>MKFTVEREHLLKPLQQVSGPLGGRPTLPILGNLLLQVADGTLSLTGTDLEMEMVARVALVQPHEPGATTVPARKFFDICRGLPEGAEIAVQLEGERMLVRSGRSRFSLSTLPAADFPNLDDWQSEVEFTLPQATMKRLIEATQFSMAHQDVRYYLNGMLFETEGEELRTVATDGHRLAVCSMPIGQSLPSHSVIVPRKGVIELMRMLDGGDNPLRVQIGSNNIRAHVGDFIFTSKLVDGRFPDYRRVLPKNPDKHLEAGCDLLKQAFARAAAASNEKFRGVRLYVSENQLKITANNPEQEEAEEILDVTYS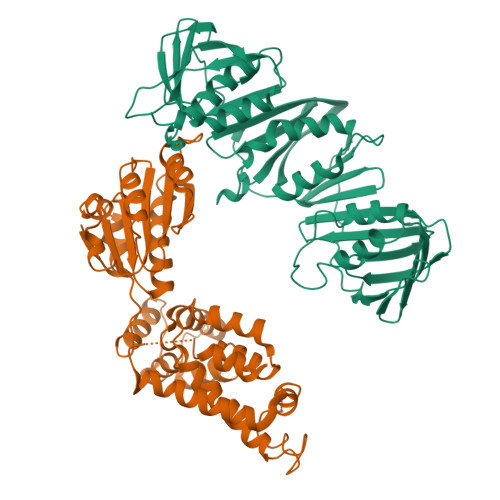GAEMEIGFNVSYVLDVLNALKCENVRMMLTDSVSSVQIEDAASQSAAYVVMPMRL[2x];>[2x]MIRLYPEQLRAQLNEGLRAAYLLLGNDPLLLQESQDAVRQVAAAQGFEEHHTFSIDPNTDWNAIFSLCQAMSLFASRQTLLLLLPENGPNAAINEQLLTLTGLLHDDLLLIVRGNKLSKAQENAAWFTALANRSVQVTCQTPEQAQLPRWVAARAKQLNLELDDAANQVLCYCYEGNLLALAQALERLSLLWPDGKLTLPRVEQAVNDAAHFTPFHWVDALLMGKSKRALHILQQLRLEGSEPVILLRTLQRELLLLVNLKRQSAHTPLRALFDKHRVWQNRRGMMGEALNRLSQTQLRQAVQLLTRTELTLKQDYGQSVWAELEGLSLLLCHKPLADVFIDG> EVARVRNLNRIIMGKYEIEPWYFSPYPIELTDEDFIYIDDFTLQYFGSKKQYERYRKKCTLRHPPGNEIYRDDYVSFFEIDGRKQRTWCRNLCLLSKLFLDHKTLYYDVDPFL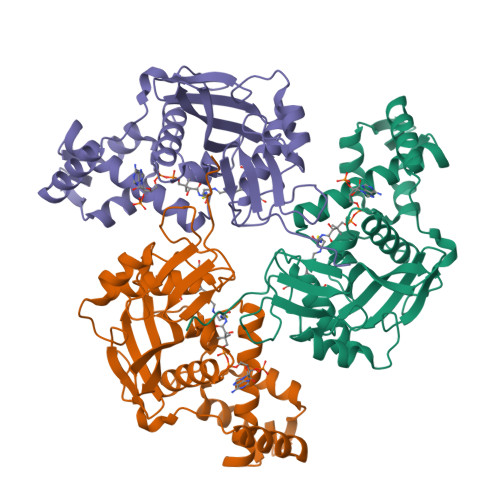FYCMTRRDELGHHLVGYFSKEKESADGYNVACILTLPQYQRMGYGKLLIEFSYELSKKENKVGSPEKPLSDLGLLSYRAYWSDTLITLLVEHQKEITIDEISSMTSMTTTDILHTAKTLNILRYYKGQHIIFLNEDILDRYNRLKAKKRRTIDPNRLIWKPPV;> GKGGAKRHRKIL To address this challenge, we develop a computational “anchor extension” methodology for targeting protein interfaces by extending a peptide chain around a non-canonical amino acid residue anchor. To test our approach using a well characterized model system, we design cyclic peptides that inhibit histone deacetylases 2 and 6 (HDAC2 and HDAC6) with enhanced potency compared to the original anchor (IC50 values of 9.1 and 4.4 nM for the best binders compared to 5.4 and 0.6 µM for the anchor, respectively). SHA can coordinate to the zinc ion in the active site of HDACs. In all the crystal structures we obtained, the thiol functional group of SHA coordinates the catalytic Zn2+ ion with a Zn2+– S separation of 2.3 Å in a distorted tetrahedral geometry reminiscent of that observed for the inhibitor Largazole.

Our first computational method (design method 1) started with docking structured cyclic-peptide scaffolds onto SHA and re-designing the residues in the interface to improve binding. We selected docked poses without clashes between the macrocycle backbone and HDAC2, and then redesigned the peptide sidechains using Rosetta combinatorial sequence optimization to maximize predicted affinity for the HDAC2. Tens of thousands of conformers were generated for each of the 100 peptides, their energies were evaluated, and those designs for which the designed target structure had the lowest energy were selected for downstream analysis. From the previous pool, five peptides with the greatest in silico predicted affinities were tested for HDAC2 inhibition in vitro, the best of which (des1.1.0) demonstrated an IC50 value of 289 nM. The crystal structure of this design in complex with HDAC2 revealed two distinct binding modes and peptide conformations in the three protein chains of the asymmetric unit, suggesting flexibility of the peptide as well as presence of iso-energetic binding conformations. In two of the protein chains of the asymmetric unit (chains B and C), the peptide conformation was very similar to the design model, but the observed binding mode to HDAC2 differed from that of the design model. This binding orientation interacts with several water molecules through backbone-mediated hydrogen bonds. In the des1.1.0:HDAC2 co-crystal structure, the dominant binding mode in the crystal (chains B and C) has considerably better predicted affinity than the original design model with the same peptide structure. Thus, the lack of structure recapitulation in this case was due to insufficient sampling—our original design calculations were not extensive enough to identify this lower energy alternative state. We found that a large-scale parallel docking algorithm which allows movements of side-chains and backbone of the peptide and nearby protein residues can reproduce the overall peptide behavior in the binding pocket for this design.

>[3x]AAYSQGGGKKKVCYYYDGDIGNYYYGQGHPMKPHRIRMTHNLLLNYGLYRKMEIYRPHKATAEEMTKYHSDEYIKFLRSIRPDNMSEYSKQMQRFNVGEDCPVFDGLFEFCQLSTGGSVAGAVKLNRQQTDMAVNWAGGLHHAKKSEASGFCYVNDIVLAILELLKYHQRVLYIDIDIHHGDGVEEAFYTTDRVMTVSFHKYGEYFPGTGDLRDIGAGKGKYYAVNFPMRDGIDDESYGQIFKPIISKVMEMYQPSAVVLQCGADSLSGDRLGCFNLTVKGHAKCVEVVKTFNLPLLMLGGGGYTIRNVARCWTYETAVALDCEIPNELPYNDYFEYFGPDFKLHISPSNMTNQNTPEYMEKIKQRLFENLRMLPHAPGVQMQAI;>[3x]XNPKQKWG> GSWFHEGLSRHQAENLLMGKEVGFFIIRASQSSPGDFSISVRHEDDVQHFKVMRDNK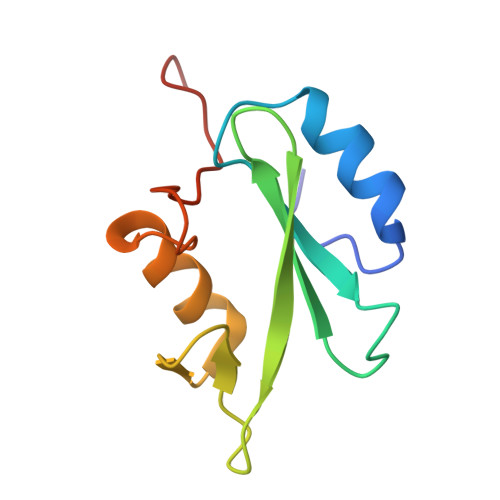GNYFLWTEKFPSLNKLVDYYRTNSISRQKQIFLRDRTREDQGH>[2x]GSTEQTAQLGTELFI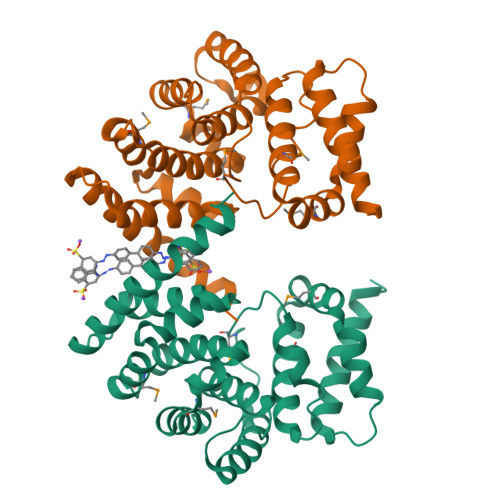VRQLLQIVKQKTNQNSVDTTLKFTLSALWNLTDESPTTCRHFIENQGLELFMRVLESFPTESSIQQKVLGLLNNIAEVQELHSELMWKDFIDHISSLLHSVEVEVSYFAAGIIAHLISRGEQAWTLSRSQRNSLLDDLHSAILKWPTPECEMVAYRSFNPFFPLLGCFTTPGVQLWAVWAMQHVCSKNPSRYCSMLIEEGGLQHLYNIKDHEHTDPHVQQIAVAILDSLEKHIVR4-bromo-5-methyl-N-[1-(3-nitropyridin-2-yl)piperidin-4-yl]-1H-pyrrole-2-carboxamide 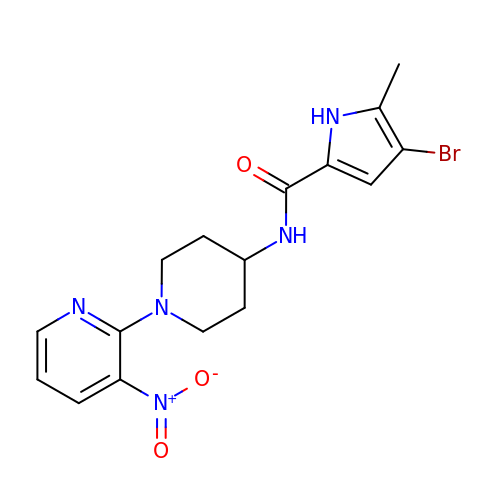| C16 H18 Br N5 O3 | AUXATGQLTJKTRN-UHFFFAOYSA-N>GSHMEAVQNRIVEAAERVPGVRGVIHLRARYVGQDIWADMIIGVDPENTVEQAHEICEAVQA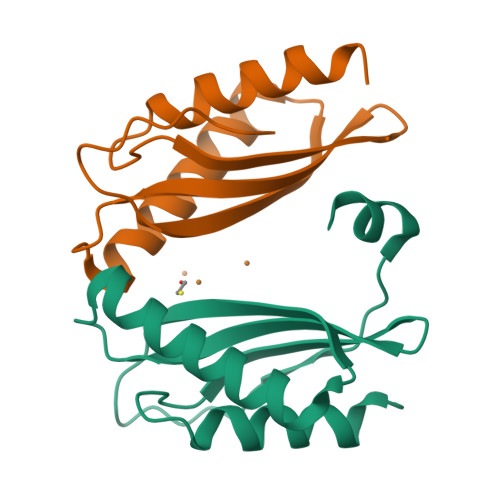AVCGKIRRIESLHVSAEAREIGDTTKPSFSDQPLSFDEVMLSKVDN[2x]> GSHMRPQGATVSLWETVQKWREYRRQCQRSLTEDPPPAT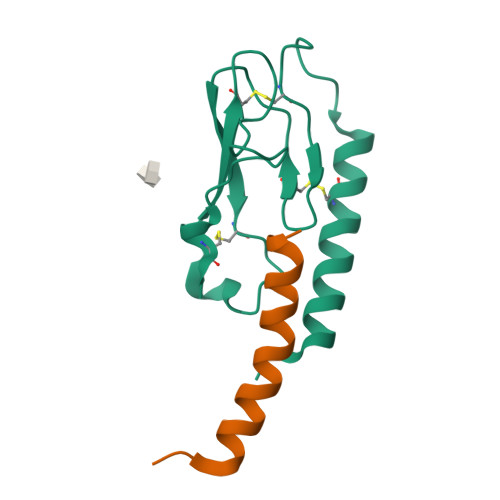DLFCNRTFDEYACWPDGEPGSFVNVSCPWYLPWASSVPQGHVYRFCTAEGLWLQKDNSSLPWRDLSECEESKRGERSSPEEQLLFLY;> HAEGTFTSDVSSYLEGQAAKEFIAWLVKGRG The adaptor protein, speckle-type BTB/POZ protein (SPOP), recruits substrates to the cullin-3-subclass of E3 ligase for selective protein ubiquitylation. SPOP recruits substrates via its N-terminal MATH domain, whereas a central BTB domain mediates dimerization and interactions with Cul3. Here, we show that MyD88 interacts with SPOP through a long degron that contains the established SPOP-binding consensus and an N-terminal site that we name the Q-motif. We determine the structural basis of these interactions and show that the Q-motif interacts with an unexplored binding pocket on the SPOP MATH domain.

To understand the structural basis of the MyD88-SPOP interaction, we solved a 1.9 Å crystal structure of SPOPMATH in complex with a MyD88 peptide, 125AEKPLQVAAVDSSVPRT141. In total, 15 residues of the 17-mer peptide were well resolved, with only Ala125 and Thr141 missing, most likely due to flexibility of these terminal regions. The MyD88 peptide binds in a groove on the surface of SPOPMATH, making extensive contacts and burying ~827 Å2 of surface area. The SBC residues interact at an edge β-strand in a manner observed in other SPOP substrates, whereas the interactions of residues located N- and C-terminal to the SBC are unique to MyD88. The side chain of MyD88 Val134 is buried in a hydrophobic pocket that is contributed by SPOP residues Phe102, Tyr123, Trp131, and Phe133, whereas the side chains of MyD88 residues 135DSS137 are involved in hydrogen bonding with the side chains of SPOP residues Tyr87, Lys129, and Asp130. MyD88 Val138 cannot make these contacts, and instead, the backbone NH group of MyD88 Arg140 forms a hydrogen bond with the side chain of SPOP Asp77, thereby directing the C-terminus of the MyD88 peptide in a different direction from that observed in other SPOP substrates. The N-terminal residues of the MyD88 peptide (127KPLQV131) form both hydrophobic- and hydrogen-bond interactions within the substrate-binding groove. The side chains of MyD88 Leu129 and Gln130 sit in a hydrophobic pocket that is contributed by SPOP residues Phe136, Ile137, and Phe141, with the side chain of Gln130 also forming hydrogen bonds with the backbone carbonyl groups of SPOP Lys115 and Phe136. This binding mode is stabilized by backbone–backbone interactions between MyD88 Leu129 and SPOP Arg138 and between MyD88 Val131 and SPOP Lys135. The side chain of SPOP Tyr83 is involved in anchoring the peptide in this region, where it forms a hydrogen bond with the backbone carbonyl group of MyD88 Pro128 and contributes hydrophobic interactions with MyD88 Pro128 and Val131.

> AKVVKFSYMWTINNFSFCREEMGEVIKSSTFSSGANDKLKWCLRVNPKGLDEESKDYLSLYLLLVSCPKSEVRAKFKFSILNAKGEETKAMESQRAYRFVQGKDWGFKKFIRRDFLLDEANGLLPDDKLTLFCEVSVVQD;> AEKPLQVAAVDSSVPRT>MSIKIRDFGLGSDLISL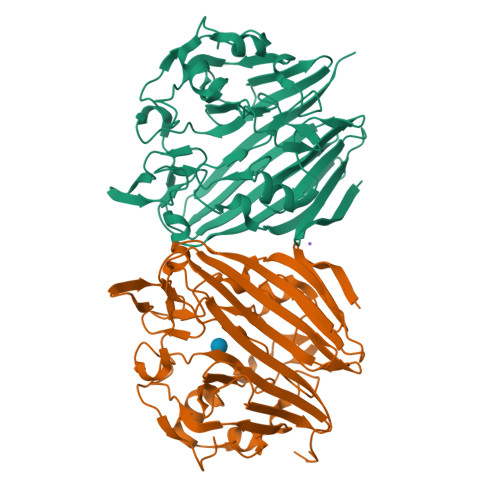TNKAGVTISFTNLGARIVDWQKDGKHLILGFDSAKEYLEKDAYPGATVGPTAGRIKDGLVKISGKDYILNQNEGPQTLHGGEESIHTKLWTYEVTDLGAEVQVKFSLVSNDGTNGYPGKIEMSVTHSFDDDNKWKIHYEAISDKDTVFNPTGHVYFNLNGDASESVENHGLRLAASRFVPLKDQTEIVRGDIVDIKNTDLDFRQEKQLSNAFNSNMEQVQLVKGINHPFLLDQLGLDKEQARLTLDDTSISVFTDQPSIVIFTANFGDLGTLYHEKKQVHHGGITFECQVSPGSEQIPELGDISLKAGEKYQATTIYSLHTKLEHHHHHH[2x]>[2x]PSAYGSVKAYTNFDAERDALNIETAIKTKGVDEVTIVNILTNRSNEQRQDIAFAYQRRTKKELASALKSALSGHLETVILGLLKTPAQYDASELKASMKGLGTDEDSLIEIICSRTNQELQEINRVYKEMYKTDLEKDIISDTSGDFRKLMVALAKGRRAEDGSVIDYELIDQDARDLYDAGVKRKGTDVPKWISIMTERSVPHLQKVFDRYKSYSPYDML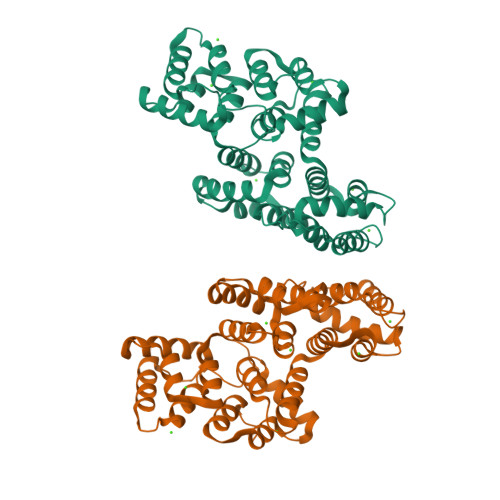ESIRKEVKGDLENAFLNLVQCIQNKPLYFADRLYDSMKGKGTRDKVLIRIMVSRSEVDMLKIRSEFKRKYGKSLYYYIQQDTKGDYQKALLYLCGGDD> GLGDLIEGVVEGVTRNALTPLTPANNLPDTQSSGPAHSKETPALTAVETGATNPLVPSDTVQTRHVIQKRTRSESTVESFFARGACVAIIEVDNDAPTKRASKLFSIWKITYKDTVQLRRKLEFFTYSRFDMELTFVVTSNY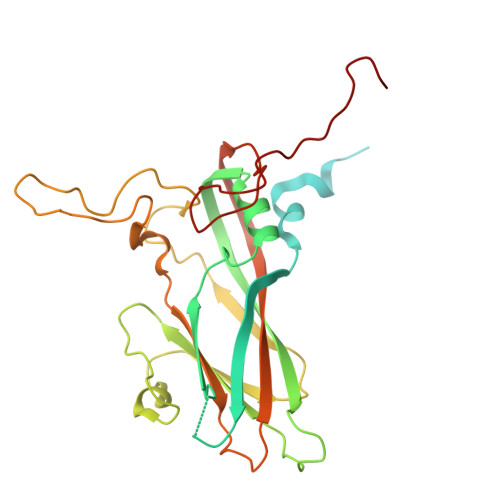TDANNGHALNQVYQIMYIPPGAPIPGKWNDYTWQTSSNPSLFYTYGAPPARISVPYVGIANAYSHFYDGFAKVPLAGQASTEGDSLYGAASLNDFGSLAVRVVNDHNPTKLTSKIRVYMKPKHVRVWCPRPPRAVPYYGPGVDYKDGLAPLPEKGLTTY>MFTGSIVAIVTPMDEKGNVCRASLKKLIDYHVASGTSAIVSVGTTGESATLNHDEHADVVMMTLDLADGRIPVIAGTGANATAEAISLTQRFNDSGIVGCLTVTPYYNRPSQEGLYQHFKAIAEHTDLPQILYNVPSRTGCDLLPETVGRLAKVKNIIGIKEATGNLTRVNQIKELVSDDFVLLSGDDASALDFMQYGGHGVISVTANVAARDMAQMCKLAAEGHFAEARVINERLMPLHNKLFVEPNPIPVKW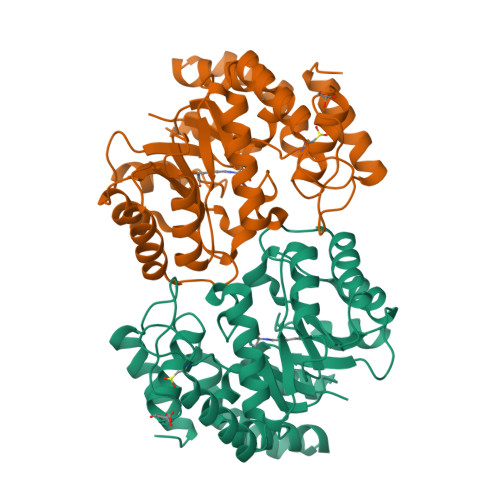ACKELGLVATDTLRLPMTPITDSGRETVRAALKHAGLL[2x]>[2x]AQKSV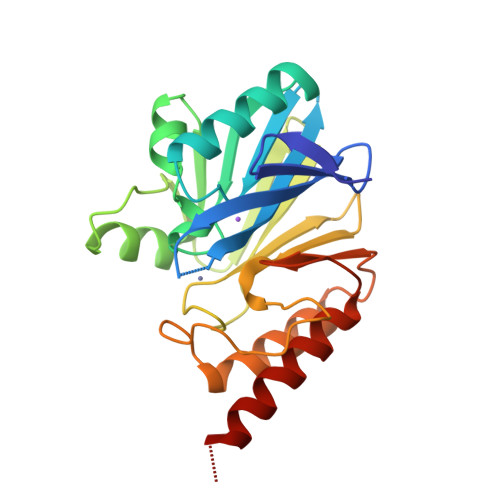KISDDISITQLSDKVYTYVSLAEIEGWGMVPSNGMIVINNHQAALLDTPINDAQTETLVNWVADSLHAKVTTFIPNHWHGDCIGGLGYLQKKGVQSYANQMTIDLAKEKGLPVPEHGFTDSLTVSLDGMPLQCYYLGGGHATDNIVVWLPTENILFGGCMLKDNQATSIGNISDADVTAWPKTLDKVKAKFPSARYVVPGHGDYGGTELIEHTKQIVNQYIESTSKP>[8x]MGCGIMKYGITEMVKTIDTKTRVVDVTNEIAKKKYQAIRDFLEGEEFKEVVIFGVYLWGNYTAQMLSKYADKVYLVDIHEFMKGFVPNNNSIKFLNLNEFKLKFIRGEVNPDLIVDLTGLGGIEPEFLAKFNPKVFIVEDPKGVFDVDIYEADNTYKRTAPFIEKAKVGV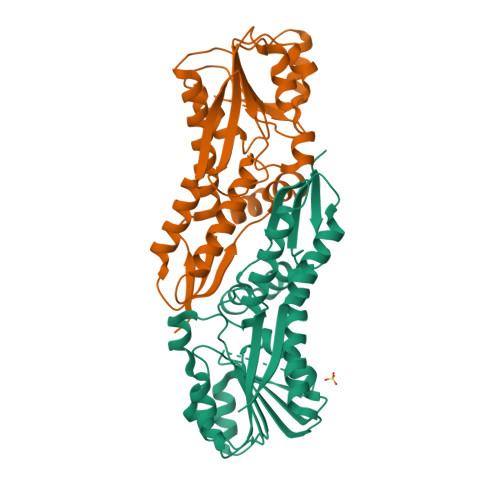LKTYRKARVSKTSGTMTLTIDTIVDASREITSLDGVLYAIPNLRYYEGILFHENDIHKFLSEISQPAITISTLNDVLDEAEEILSNNINLIYSFVEEL> GAMGSTSLEPTSTLVRVRKSAAT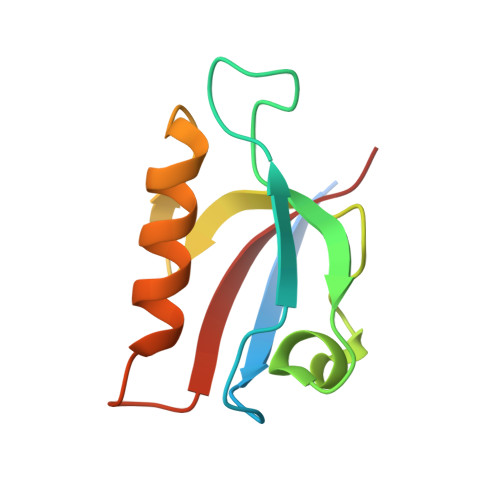LGIAIEGGANTRQPLPRIVTIQRGGSAHNCGQLKVGHVILEVNGQTLRGKEHKEAARIIAEAFKTKERDYIDFLVTEFN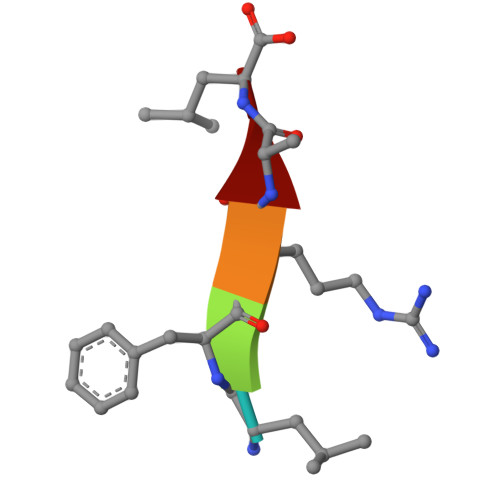> LFRAL>GSPGIPGSTRMAYQHCPFDTLLILDFETTSDAANQDYPCEVIQFAIVAYDVPNDKIREDISFNKYVKPVLNRTLTKNCVDFTGIPQRSIDTADTFDVVYEQFQQWLITLGLEEGKFAFVCDSRQDLWRIAQYQMKLSNIQMPAFFRQYINLYKIFTNEMDRMGPKELSATTNIGKMNEYYDLPTIGRAHDAMDDCLNIATILQRMINMGAKVTVNELLTCCASWRRQPLVYNKEWRSSFMDAGKIFERVLPLVVTTI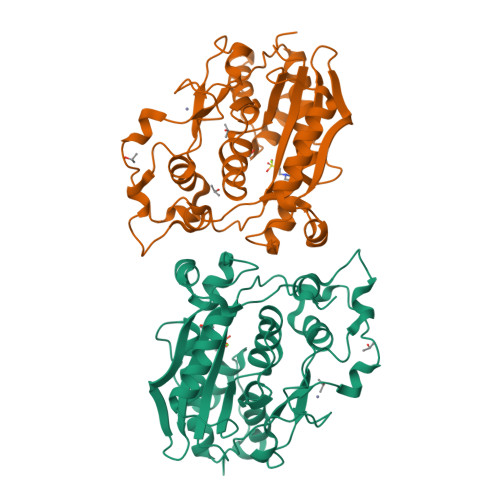RAGDFRLEMYGVCRYCRKGMDVCGTSHQQTPHDLYKNEEDPIHFAKIAGYY[2x]> MEHQLLCCEVETIRRAYPDANLLNDRVLRAMLKAEETCAPSVSYFKCVQKEVLPSMRKIVATWMLEVCEEQKCEEEVFPLAMNYLDRFLSLEPVKKSRLQLLGATCMFVASKMKETIPLTAEKLCIYTDNSIRPEELLQMELLLVNKLKWNLAAMTPHDFIEHFLSKMPEAEENKQIIRKHAQTFVALCATDVKFISNPPSMVAAGSVVAAVQGLNLRSPNNFLSYYRLTRFLSRVIKCDPDCLRACQEQIEALLESSLRQAQQNMDPKAA;> MATSRYEPVAEIGVGAYGTVYKARDPHSGHFVALKSVRVPNGEEGLPISTVREVALLRRLEAFEHPNVVRLMDVCATSRTDREIKVTLVFEHVDQDLRTYLDKAPPPGLPAETIKDLMRQFLRGLDFLHANCIVHRDLKPENILVTSGGTVKLADFGLARIYSYQMALDPVV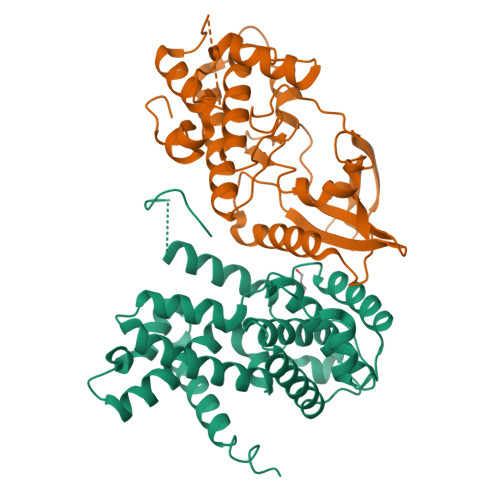VTLWYRAPEVLLQSTYATPVDMWSVGCIFAEMFRRKPLFCGNSEADQLGKIFDLIGLPPEDDWPRDVSLPRGAFPPRGPRPVQSVVPEMEESGAQLLLEMLTFNPHKRISAFRALQHSYLHKDEGNPEHHHHHH>[5x]MAELPPGRLATTEDYFAQQAKQAVTPDVMAQLAYMNYIDFISPFYSRGCSFEAWELKHTPQRVIKYSIAF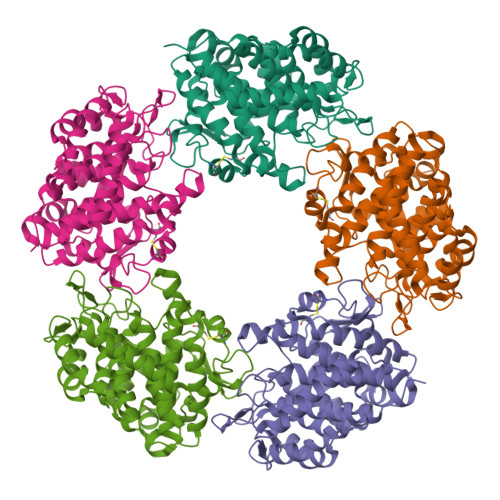YAYGLASVALIDPKLRALAGHDLDIAVSKMKCKRVWGDWEEDGFGTDPIEKENIMYKGHLNLMYGLYQLVTGSRRYEAEHAHLTRIIHDEIAANPFAGIVAEPDNYFVQCNSVAYLSLWVYDRLHGTDYRAATRAWLDFIQKDLIDPERGAFYLSYHPESGAVKPWISAYTTAWTLAMVHGMDPAFSERYYPRFKQTFVEVYDEGRKARVRETAGTDDADGGVGLASAFTLLLAREMGDQQLFDQLLNHLEPPAKPSIVSASLRYEHPGSLLFDELLFLAKVHAGFGALLRMPPPAAKLAGK>MYGLVNKAIQDMISKHHGEDTWEAIKQKAGLEDIDFFVGMEAYSDDVTYHLVGAASEVLGKPAEELLIAFGEYWVTYTSEEGYGELLASAGDSLPEFMENLDNLHARVGLSFPQLRPPAFECQHTSSKSMELHYQSTRAGLAPMVLG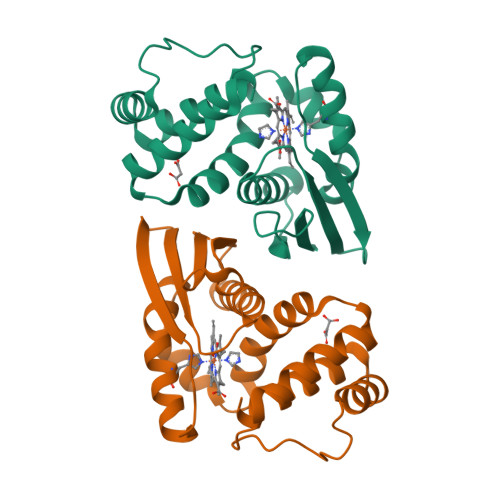LLHGLGKRFQTKVEVTQTAFRETGEDHDIFSIKYE[2x]>MA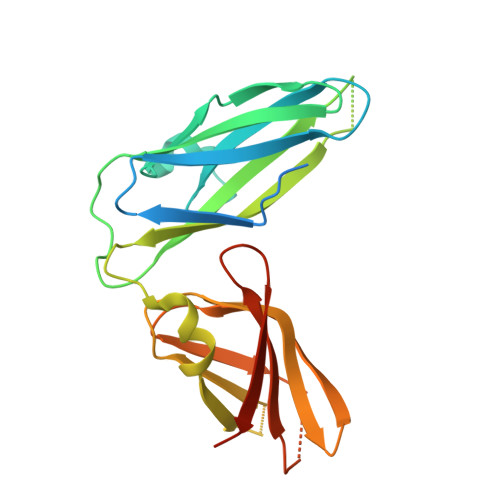PLMHRFHSFVAASAVAIALCVGTAHAGLIAQGTRVVFPASEREVTLRVSNTSGTPVLAQAWIDDGRQDVPPEELQVPFSVTPAVTRVEPNGGAVLRIAYLKAPLPTDRESLFWLNILEVPPRDEDENNALQFSFRSRFKLFFRPSQLKSVDSAAGKLQWKFLESGGAGKKTVVQVNNPTPYYVSFASVELIVDGRVMSVGKGMVAPFSTKEFDWQGNPKNMEAASVRYEVINDYGGRNTHDRALGKRGSHHHHHH[2x]>SMGSRYAVKLDTDFDNPKWIARHKHMFNFLDINSNGQINLNEMVHKASNIICKKLGATEEQTRRHQKCVEDFFGGAGLEYDKDTTWPEYIEGWKRLAKTELERHSKNRVTLIRLWGDALFDIIDKDGNGSVSLDEWIQYTHCAGIQQSRGQCEATFAHCDLDGDGKL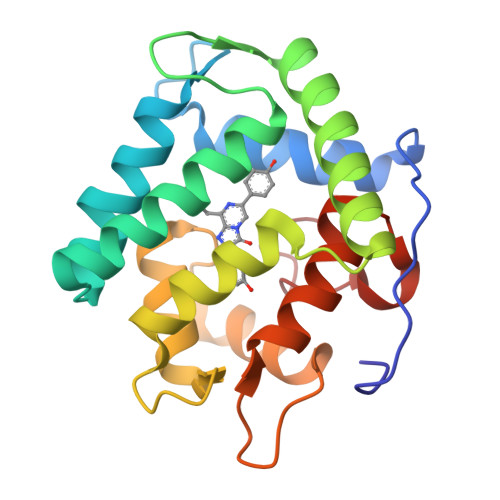DVDEMTRQHLGFWYSVDSTCEGLYGGAVPY[2x]> QFAKPEDAVKYRQSALTLMASHFGRMTPVVKGQAPYDAAQIKAN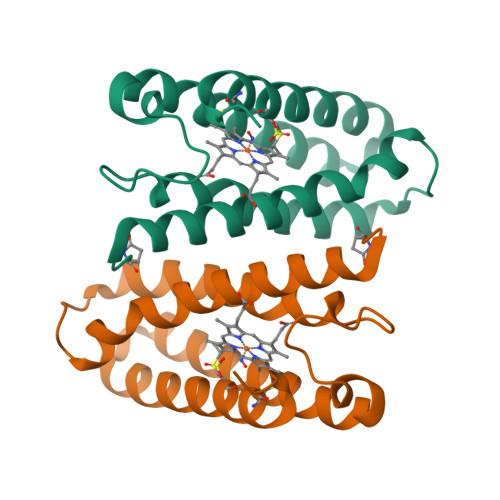VEVLKTLSALPWAAFGPGTEGGDARPEIWSDAASFKQKQQAFQDNIVKLSAAADAGDLDKLRAAFGDVGASCKACHDAYKKKK2-deoxy-2-fluoro-alpha-D-glucopyranose | 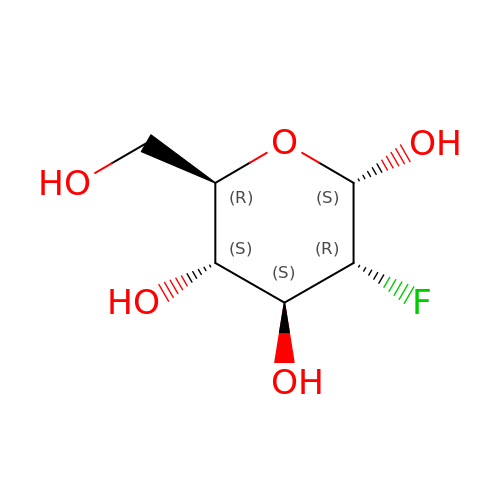C6 H11 F O5 | ZCXUVYAZINUVJD-UKFBFLRUSA-N>AVSKVYARSVYDSRGN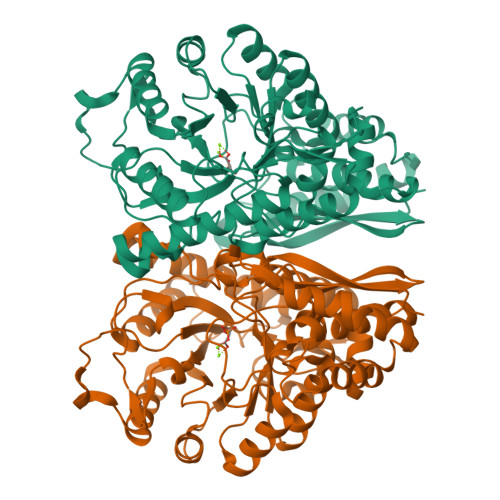PTVEVELTTEKGVFRSIVPSGASTGVHEALEMRDGDKSKWMGKGVLHAVKNVNDVIAPAFVKANIDVKDQKAVDDFLISLDGTANKSKLGANAILGVSLAASRAAAAEKNVPLYKHLADLSKSKTSPYVLPVPFLNVLNGGSHAGGALALQQFMIAPTGAKTFAEALRIGSEVYHNLKSLTKKRYGASAGNVGDEGGVAPNIQTAEEALDLIVDAIKAAGHDGKVKIGLDCASSEFFKDGKYDLDFKNPNSDKSKWLTGPQLADLYHSLMKRYPIVSIEDPFAEDDWEAWSHFFKTAGIQIVADDLTVTNPKRIATAIEKKAADALLLKVNQIGTLSESIKAAQDSFAAGWGVMVSHRSGETEDTFIADLVVGLRTGQIKTGAPARSERLAKLNQLLRIEEELGDNAVFAGENFHHGDKL[2x]> MVRNQRYPASPVQEIFLPEPVPFVQFDQTAPSPNSPPAPLPSPSLSQCEEQKDRYRDISSMFHRGVAGAEQVREAYNSMAKCFRRVSVAEVLESDPAFRQARNFTMDLKQAEDDQRYKQ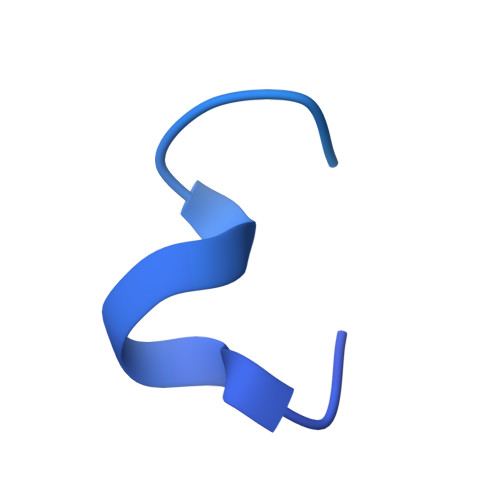LQYGRVPSILTKYHL> GWKTNKYGTLYKSESASFTPNTDIITRTTGPFRSM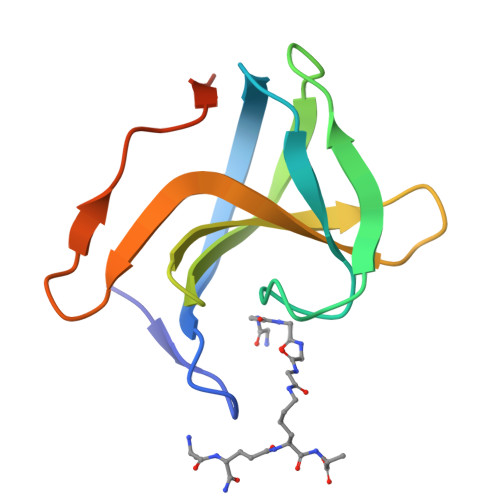PQSGVLKAGQTIHYDEVMKQDGHVWVGYTGNSGQRIYLPVRTWNKSTNTLGVLWGTIKVLWGTIK> MGSSHHHHHHSGLVPRGSHMATPPKRSSPSFSASSEGTRIKKISIEGNIAAGKSTFVNILKQLSEDWEVVPEPVARWSNVQSTQDEFEELTMSQKNGGNVLQMMYEKPERWSFTFQTYACLSRIRAQLASLNGKLKDAEKPVLFFERSVYSDRYIFASNLYESESMNETEWTIYQDWHDWM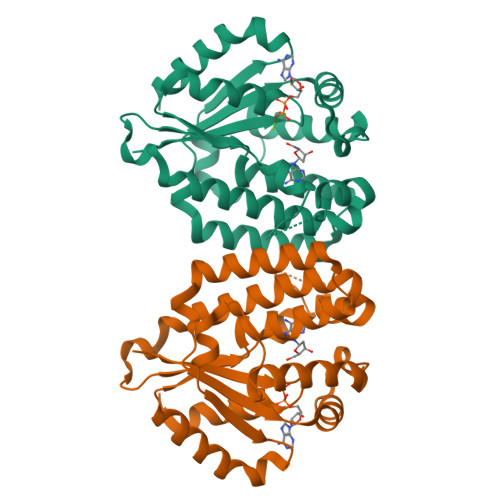NNQFGQSLELDGIIYLQATPETCLHRIYLRGRNEEQGIPLEYLEKLHYKHESWLLHRTLKTNFDYLQEVPILTLDVNEDFKDKYESLVEKVKEFLSTL benzoyl-oxydephosphocoenzyme A | C28 H39 N7 O15 P2 | 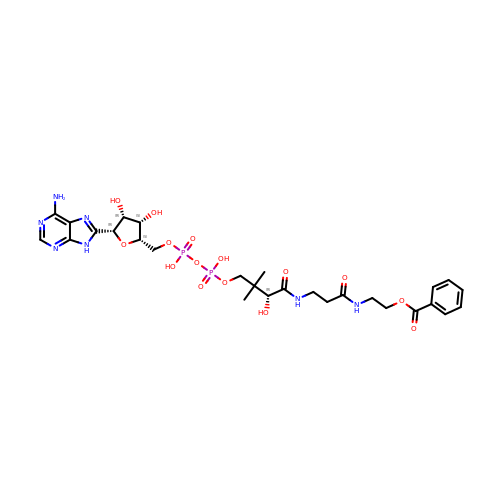KLLSEACSJWFZEP-NKRQLCBBSA-N>[4x]GAMSAADEVDGLGVARPHYGS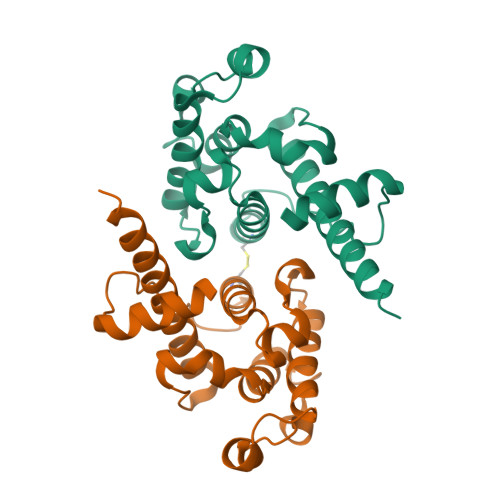VLDNERLTAEEMDERRRQNVAYEYLCHLEEAKRWMEACLGEDLPPTTELEEGLRNGVYLAKLGNFFSPKVVSLKKIYDREQTRYKATGLHFRHTDNVIQWLNAMDEIGLPKIFYPETTDIYDRKNMPRCIYCIHALSLYLFCLGLAPQIQDLYGKVDFTEEEINNMKTELEK> MTDFYTIKDAQADLAIAPLNLTVLLAPYSTTPATTLESPTDGSLAIPPGYKSVGHFEKQAGLTLGNEFDSKDIEAYGEPEPIRTIINKRTTTFDFAMYQNQRNVLELIWTQDFSNIQPSEFGGIVLEAPKVPKNIYYRAILVGMDDRNDRPIWLYWLMPKVKLDKLDNQTLNDDNVIEYKPTLKAFRDDVVGYSVAQGFAGPGWRDLVATAGFGEA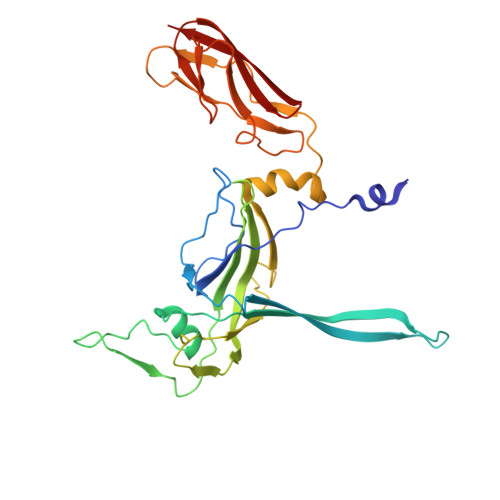LTALTITPGSPTVTVATGASHTAQLLVEGDNGINYTPDVVFTSSAPDKASVSAAGLVTGVAAGSATITATKGALTATATVTVTA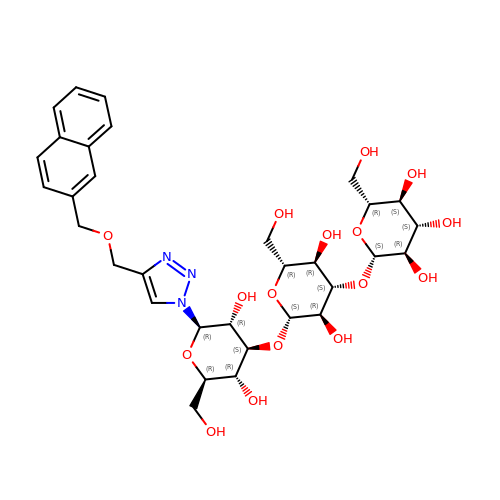(2~{R},3~{S},4~{S},5~{R},6~{S})-2-(hydroxymethyl)-6-[(2~{R},3~{R},4~{S},5~{R},6~{S})-2-(hydroxymethyl)-6-[(2~{R},3~{R},4~{S},5~{R},6~{R})-2-(hydroxymethyl)-6-[4-(naphthalen-2-ylmethoxymethyl)-1,2,3-triazol-1-yl]-3,5-bis(oxidanyl)oxan-4-yl]oxy-3,5-bis(oxidanyl)oxan-4-yl]oxy-oxane-3,4,5-triol | C32 H43 N3 O16 | INTPLNBRTDNBOM-DGUZUYFASA-N>CCAGTACTGG[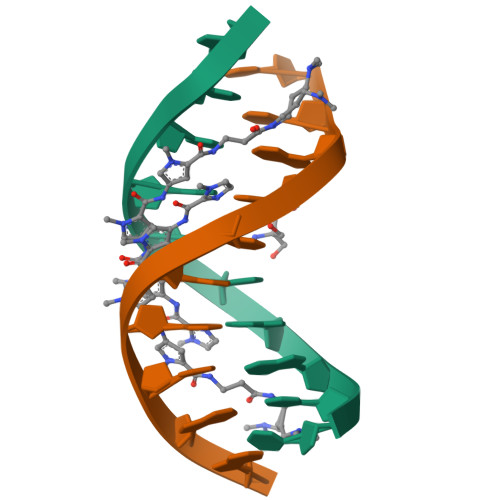2x]>[2x]MSLKITEVKAHALSTPIPERMRVESGAGLKLNRQMILVEVRTDEGVTGVGSPSGPYDLAVLKRAIEDVIGPQLIGEDPANINYLWHKVFHGEVSRNLGHRSVGIAAMSGVDIALWDLKGRAMNQPIYQLLGGKFHTRGVRAYASSIYWDLTPDQAADELAGWVEQGFTAAKLKVGRAPRKDAANLRAMRQRVG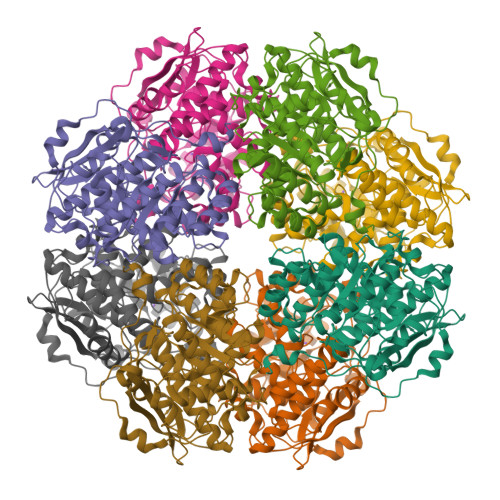ADVEILVDANQSLGRHDALAMLRILDEAGCYWFEEPLSIDDIEGHRILRAQGTPVRIATGENLYTRNAFNDYIRNDAIDVLQADASRAGGITEALAISASAASAHLAWNPHTFNDIITVAANLHLVAASPHPAMFEWDITHNDLMTRLASYDLKLENGLVQPPQGPGLGFEIDWDFVAAHAWKGEPAIGAGHGMKKEGHHHHHH N-adamantan-2-yl-1-ethyl-D-prolinamide | C17 H28 N2 O 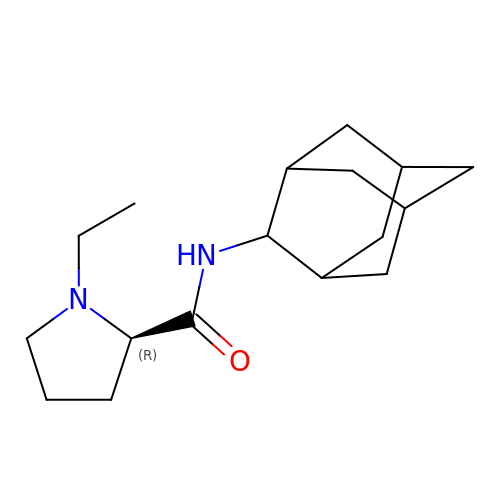| UJRJQNDIYCDCNX-ZTYXSZCMSA-N>[2x]SQIGLFSKICRVTIKTLHYYNKIGLLVPAYINPDNGYRFYTSDQLMKFHQIASLRQLGFTITEIVTLTQDENSCHIIERRRLEIQKQIRDMADMLSRINHYLQHKKKERIMLYQAALKEIPECIVYSKRFIVPDFSSYIKLIPPIGQEVMKANPGLTLTTPAYCFTLYHDKEYKEKNMDVEFCEAVNDFGKNEGNIIFQVIPAITAVTVIHKGPYDSLRNAYIYLMQWVEDNGYLLTNSPRESYIDGIWNKQDSAEWMTEIQFPVEKV

Bacterial RNA polymerase (RNAP) holoenzyme initiates transcription by recognizing the conserved –35 and –10 promoter elements that are optimally separated by a 17-bp spacer. The MerR family of transcriptional regulators activate suboptimal 19–20 bp spacer promoters in response to myriad cellular signals, ranging from heavy metals to drug-like compounds. Here we report one crystal structure of a multidrug-sensing MerR family regulator EcmrR and nine cryo-electron microscopy structures that capture the EcmrR-dependent transcription process from promoter opening to initial transcription to RNA elongation. These structures reveal that EcmrR is a dual ligand-binding factor that reshapes the suboptimal 19-bp spacer DNA to enable optimal promoter recognition, sustains promoter remodeling to stabilize initial transcribing complexes, and finally dissociates from the promoter to reverse DNA remodeling and facilitate the transition to elongation.

When including ribonucleoside triphosphates (rNTPs) in the complexes (see METHOD DETAILS), we obtained two structures of the RNAP-promoter initial transcribing complexes (RPitc) containing either a 3-nt de novo synthesized RNA transcript on the heteroduplex DNA scaffold (hereinafter designated EcmrR-RPitc-3nt) or a 4-nt RNA transcript on a fully complementary DNA scaffold (hereinafter designated EcmrR-RPitc-4nt). Unlike site I, which is occupied by TPSb+ in all of the three EcmrR-RNAP-promoter complexes, site II in EcmrR-RPitc-3nt is vacant when CHAPSO was omitted during sample preparation, indicating that site II might have different selectivity for ligands compared with site I and that its occupancy is not essential for EcmrR-mediated transcription activation. In comparison, site II is relatively flexible and undergoes significant conformational changes between its un-liganded, CTA+-bound and CHAPSO-bound forms. Y174 and R220, which partially occupy site II in the absence of ligand, gradually lift up as a ligand binds and as the bound ligand gets bulkier.>GVFKVMLVGESGVGKSTLAGTFGGLQGDHAHEMENSEDTYERRIMVDKEEVTLIVYDIWEQGDAGGWLQDHCLQTGDAFLIVFSVTDRRSFSKVPETLLRLRAGRPHHDLPVILVGNKSDLARSREVSLEEGRHLAGTLSCKHIETS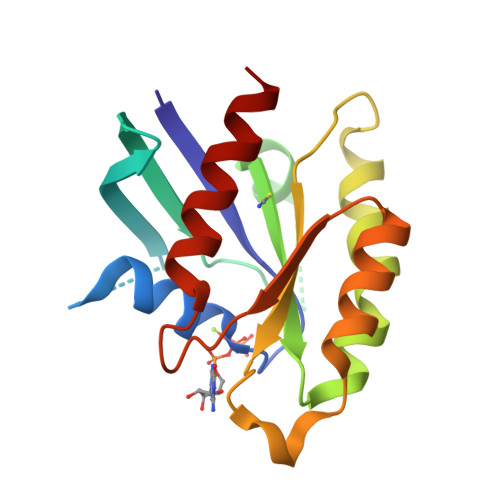AALHHNTRELFEGAVRQIRLRR[2x]>GPGMAAFVKENHRQLQARMGDLKGV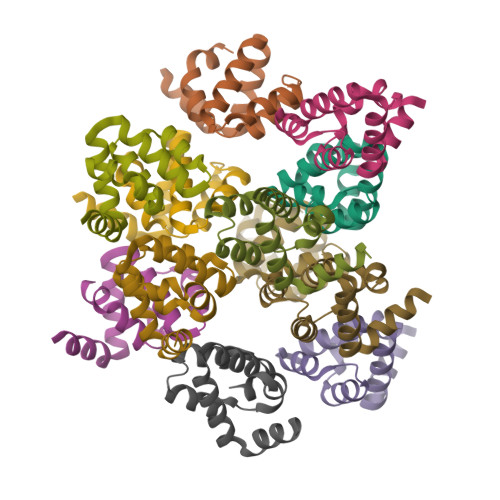LDDLQDNEVLTENEKELVEQEKTRQSKNEALLSMVEKKGDLALDVLFRSISERDPYLVSYLRQQNL[12x]Endolysins are produced by many double stranded DNA bacteriophages to effect the release of new virions from an infected cell by degrading the bacterial cell wall. Endolysins typically consist of a peptidoglycan hydrolase domain and a C-terminal domain that is often termed as a cell wall binding domain. Here, we present the crystal structures of autoproteolytic fragments of the CD27L and CTP1L endolysins, covering the C-terminal domain. We propose that the cleavage and oligomerization are linked, and they provide the endolysin with a trigger and release mechanism that leads to activation.

SDS-PAGE analysis confirmed that purified CTP1L wild type endolysin undergoes cleavage of the C-terminal domain. We then transferred the critical mutation that affected CD27L cleavage, involving the stem of the linker of the C-terminal domain of CTP1L (V195P). The SDS-PAGE analysis of purified recombinant CTP1L shows a reduction in cleavage for the V195P mutant. We attempted to crystallize the CTP1L V195P mutant to see if this slowly cleaving mutant would yield crystals of the full length protein. After 2 weeks, crystals appeared, an X-ray data set was collected to 2.1 Ångstrom and the structure of the C-terminal domain was solved by molecular replacement using the C-terminal domain of CD27L as a search model. As with CD27L, there was no N-terminal domain present in the crystal lattice. The C-terminal domain is truncated at Pro195, and there is only one molecule present in the asymmetric unit. The fold of the C-terminal domain of CTP1L is very similar to that of CD27L, except that the second alpha helix α2 is deleted, and the alpha helix α3 is extended in CTP1L. The head-on dimer is also present in the crystal lattice of the C-terminal domain of CTP1L. There is a similar side-by-side dimer present in the crystal lattice of the CTP1L C-terminal fragment, but the domains point in opposite directions compared to the same dimer observed in CD27L.

> PENLVVYNDGADQRAAEYLADRLACPTINNARKFDYSNVKNVYAVGGNKEQYTSYLTTLIAGSTRYTTMQAVLDYIKNLK>[4x]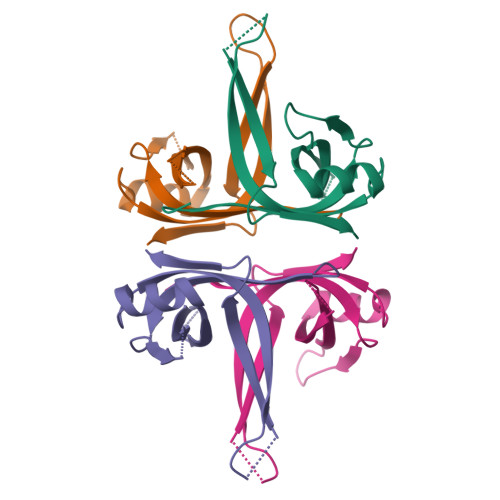MASRGVNKVILVGNLGQDPEVRYMPNGGAVANITLATSESWRDKATGEMKEQTEWHRVVLFGKLAEVASEYLRKGSQVYIEGQLRTRKWTDQSGQDRYTTEVVVNVGGTMQML>[8x]MAEKPKLHYSNIRGRMESIRWLLAAAGVEFEEKFIKSAEDLDKLRNDGYLM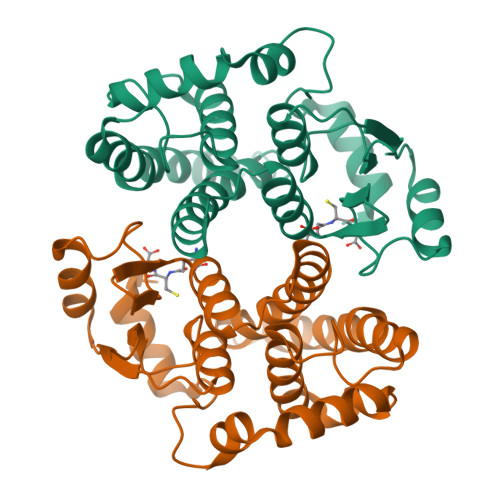FQQVPMVEIDGMKLVQTRAILNYIASKYNLYGKDIKEKALIDMYIEGIADLGEMILLLPFTQPEEQDAKLALIQEKTKNRYFPAFEKVLKSHGQDYLVGNKLSRADIHLVELLYYVEELDSSLISSFPLLKALKTRISNLPTVKKFLQPGSPRKPPMDEKSLEESRKIFRF>[2x]SSKMSDVKCTSVVLLSVLQQLRVESSSKLWAQCVQLHNDILLAKDTTEAFEKMVSLLSVLLSMQGAVDINKLCEEMLDNRATLQ;>AIASEFSSLPSYAAFATAQEAYEQAVANGDSEVVLKKLKKSLNVAKSEFDRDAAMQRKLEKMADQAMTQMYKQARSEDKRAKVTSAMQTMLFTMLRKLDNDALNNIINNARDGCVPLN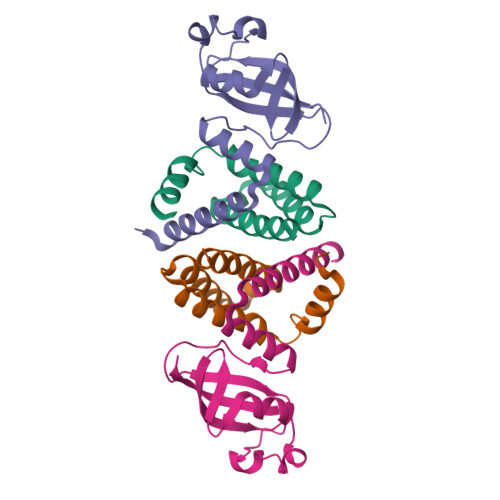IIPLTTAAKLMVVIPDYNTYKNTCDGTTFTYASALWEIQQVVDADSKIVQLSEISMDNSPNLAWPLIVTALRANSAVKLQ[2x]>[4x]SMQGPRTRARLGANEVLLVVGGFGSQQSPIDVVEKYDPKTQEWSFLPSITRKRRYVASVSLHDRIYVIGGYDGRSRLSSVECLDYTADEDGVWYSVAPMNVRRGLAGATTLGDMIYVSGGFDGSRRHTSMERYDPNIDQWSMLGDMQTAREGAGLVVASGVIYCLGGYDGLNILNSVEKYDPHTGHWTNVTPMATKRSGAGVALLNDHIYVVGGFDGTAHLSSVEAYNIRTDSWTTVTSMTTPRCYVGATVLRGRLYAIAGYDGNSLLSSIECYDPIIDSWEVVTSMGTQRCDAGVCVLRE;>[4x]AYTVVGGPPGGPPVR

KLHL12 belongs to the BTB-BACK-Kelch family of proteins, which includes E3s such as KEAP1 (KLHL19) and gigaxonin (KLHL16). Interaction with Cullin3 is mediated by the BTB domain and a ‘3-box' motif from the BACK domain, whereas the Kelch domain mediates substrate capture. In the current work, we address this gap in understanding, by defining a consensus recognition motif ‘PGXPP' common to both substrates and co-adaptors of KLHL12.

A crystal structure of the KLHL12-DVL1 complex was subsequently solved by molecular replacement and refined at 2.38 Å resolution with four complexes in the asymmetric unit. The structure traces the Kelch domain of KLHL12 from residues 279 to 567. Overall, the DVL1 peptide was traced from Gly655 to Val663 (‘GGPPGGPPV'), allowing structural analysis of the critical ‘PGGPP' motif. The bound DVL1 peptide adopts a U-shaped turn conformation that is stabilized by weak intramolecular hydrogen bonds between the carbonyl of Pro657 and the amides of Gly659 and Gly660. This conformation allows DVL1 to form interactions with all six blades of the KLHL12 β-propeller, as shown in figure 4a and b. The first proline in this motif, Pro658, forms the only hydrogen bond in the complex interface through the hydroxyl of KLHL12 Tyr512. Pro658 and the flanking residues Pro657 and Gly659 additionally contribute extensive hydrophobic interactions with KLHL12 residues Tyr321, Leu371, Tyr434, Ile439 and Phe481, which span blades III, IV, V and VI. Further hydrophobic contacts are provided by the downstream residue Pro661, which inserts between KLHL12 Phe289, Tyr528 and Leu533. Here, DVL1 Pro661 and KLHL12 Tyr528 form a prolyl-aromatic ring–ring stacking interaction. Despite the different crystal packing, the structure of KLHL12 in the DVL1 complex is unchanged compared to the unbound Kelch domain structure (0.99 Å RMSD for all atoms).> GPGSNCGPPPTLSFAAPMDITLTETRFKTGTTLKYTCLPGYVRSHSTQTLTCNSDGEWVYNTFCIYKRCRHPGELRNGQVEIKTDLSFGSQIEFS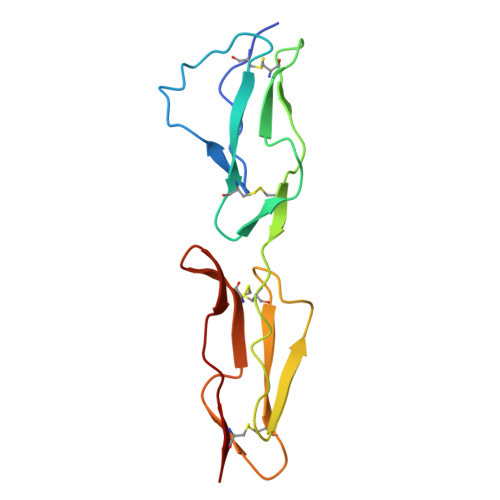CSEGFFLIGSTTSRCEVQDRGVGWSHPLPQCEI>[2x]MNHKVHHHHHHIEGRHMKVLILGAGNIGRAIAWDLKDEFDVYIGDVNNENLEKVKEFATPLKVDASNFDKLVEVMKEFELVIGALP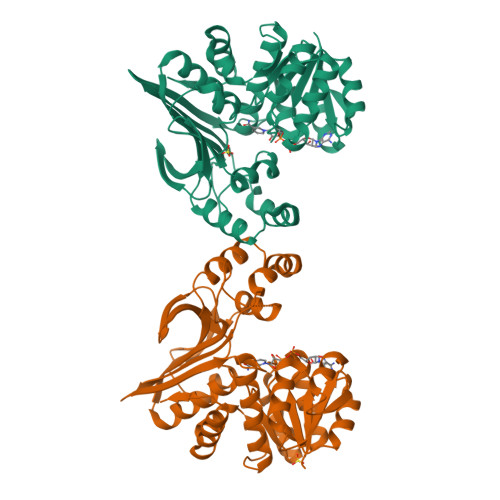GFLGFKSIKAAIKSKVDMVDVSFMPENPLELRDEAEKAQVTIVFDAGFAPGLSNILMGRIFQELDLKEGYIYVGGLPKDPKPPLYYKITWSPRDLIEEYTRPARVIRNGKVSKVDPLSEVKKVKIGKFEFEAFISDGLRSMLETINSERLEEWTLRWPGHLEKIKVLRELGFFKPENLDFTLRVIEPLMRYETKDFSIMKVVGKGEEGEMEFFLYDEEDSMFSSMSRVTGFTAAIISRIVAENTCTFGVIPPEILGMREDTFRRIIDELKERGISIEGT> RIHNRMLRARILKLDGKDYRPEEQAAFDLLRDGLLDGISNRKSTPKLDVYSDQIVWGRSPVRIDMAGGWTDTPPYSLYSGGNVVNLAIELNGQPPLQVYVKPCKDFHIVLRSIDMGAMEIVSTFDELQDYKKIGSPFSIPKAALSLAGFAPAFSAVSYASLEEQLKDFGAGIEVTLLAAIPAGSGLGTSSILASTVLGAINDFCGLAWDKNEICQRTLVLEQLLTTGGGWQDQYGGVLQGVKLLQTEAGFAQSPLVRWLPDHLFTHPEYKDCHLLYYTGITRTAKGILAEIVSSMFLNSSLHLNLLSEMKAHALDMNEAIQRGSFVEFGRLVGKTWEQNKALDSGTNPPAVEAIIDLIKDYTLGYKLPGAGGGGYLYMVAKDPQAAVRIRKILTENAPNPRARFVEMTLSDKGFQVSRS

The bifunctional l-fucokinase/GDP-β-l-fucose pyrophosphorylase (FKP) from Bacteroides fragilis catalyzes the conversion from l-fucose to GDP-β-l-fucose. The full-length FKP (FKP-FL, 949 amino acids) exists as a tetramer in solution, but the individually prepared N-terminal domain (FKP-NTD corresponding to the sequence 1–496, also containing a SUMO tag) and C-terminal domain (FKP-CTD, the sequence 519–949) form a monomer and a dimer, respectively. FKP-NTD has a single α/β domain and a β-helix-containing domain, whereas FKP-CTD folds into two α/β domains and the linker comprises three α-helices.

Initial trials with both FKP-FL and its selenomethionine (Se–Met) derivative yielded an orthorhombic crystal form, which, however, did not contain the FL protein. Instead, it turned out to have a single FKP-CTD-like molecule as the asymmetric unit, probably a result of proteolysis. Subsequent soaking of the native crystals with fucose-1-P allowed direct observation of the binding mode of the sugar–phosphate product in the kinase active site. The refined FKP-CTD–fucose-1-P model to 2.46 Å resolution contains amino acid residues 571 to 812 and 831 to 949. Fucose-1-P is bound between the two domains. The bound product fucose-1-P in the complex crystal of FKP-CTD revealed the binding mode of l-fucose (substrate) because the structure of the sugar moiety, including β-configured C1-OH, is virtually identical. In the crystal, all free hydroxyl groups of fucose-1-P are involved in direct interactions with the protein. C2-OH is hydrogen bonded to the side chain of Asp762, C3-OH to those of Asp601 and Thr602, and C4-OH to Asp601 and Gln761. The side-chain indole group of Trp599 lies parallel to the plane of C4–C5–C6 at distances of 3.5 to 4.0 Å, apparently engaged in strong van der Waals or stacking interactions with the sugar moiety. Interestingly, an analysis of the packing in the F222 crystal of FKP-CTD also shows the same tetrameric organization despite its appearance as dimers in solution.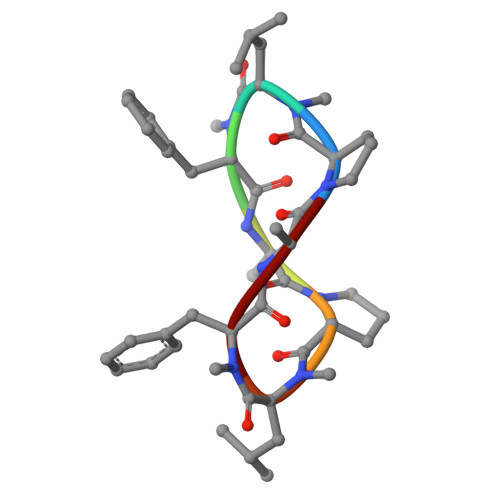> PLFAPLFA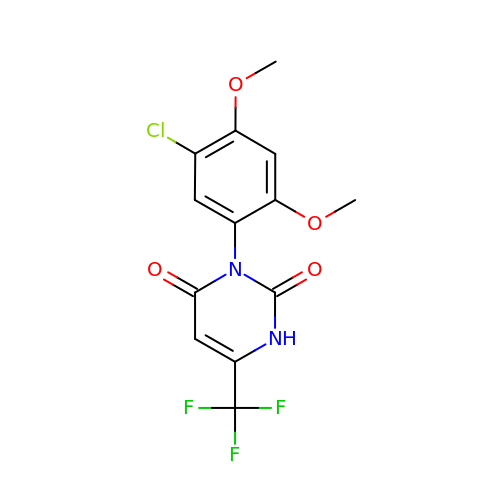3-(5-chloranyl-2,4-dimethoxy-phenyl)-6-(trifluoromethyl)-1H-pyrimidine-2,4-dione | C13 H10 Cl F3 N2 O4 | GGXGVBQCYFQKID-UHFFFAOYSA-N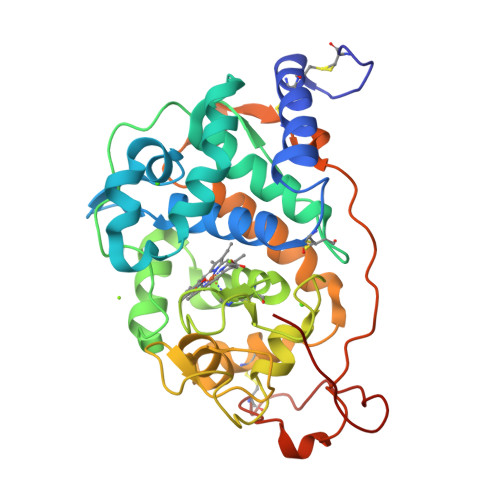> ATCDDGRTTANAACCILFPILDDIQENLFDGAQCGEEVHESLRLTFHDAIGFSPTLGGGGADGSIIAFSDIETNFPANAGIDEIVEAQKPFVAKHNISAGDFIQFAGAVGVSNCPGGVRIPFFLGRPDAVAASPDHLVPEPFDSVTSILARMGDAGFSPVEVVWLLASHSIAAADKVDPSIPGTPFDSTPGVFDSQFFIETLLKGRLFPGTADNKGEAQSPLQGEIRLQSDELLARDPRTACEWQSMVNNQPKIQNRFAATMSKMALLGQDKTKLIDCSDVIPTPPALVGAAHLPAGFSLKDVEQACAATPFPALTADPGPVTSVPPVPGS>PPYTVVYFPVRGRCAALRMLLADQGQSWKEEVVTVETWQEGSLKASCLYGQLPKFQDGDLTLYQSNTILRHLGRTLGLYGKDQQEAALVDMVNDGVEDLRCKYISLIVTNYEAGKDDYVKALPGQLKPFETLLSQNQGGKTFIVGDQISFADYNLLDLLLIHEVLAPGCLDAFPL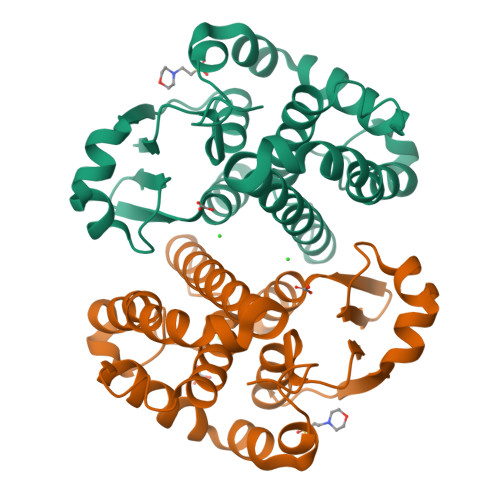LSAYVGRLSARPKLKAFLASPEYVNLPINGNGKQ[4x]> MMGHRPVLVLSQNTKRESGRKVQSGNINAAKTIADIIRTCLGPKSMMKMLLDPMGGIVMTNDGNAILREIQVQHPAAKSMIEISRTQDEEVGDGTTSVIILAGEMLSVAEHFLEQQMHPTVVISAYRKALDDMISTLKKISIPVDISDSDMMLNIINSSITTKAISRWSSLACNIALDAVKMVQFEENGRKEIDIKKYARVEKIPGGIIEDSCVLRGVMINKDVTHPRMRRYIKNPRIVLLDSSLEYKKGESQTDIEITREEDFTRILQMEEEYIQQLCEDIIQLKPDVVITEKGISDLAQHYLMRANITAIRRVRKTDNNRIARACGARIVSRPEELREDDVGTGAGLLEIKKIGDEYFTFITDCKDPKACTILLRGASKEILSEVERNLQDAMQVCRNVLLDPQLVPGGGASEMAVAHALTEKSKAMTGVEQWPYRAVAQALEVIPRTLIQNCGASTIRLLTSLRAKHTQENCETWGVNGETGTLVDMKELGIWEPLAVKLQTYKTAVETAVLLLRIDDIVSGHKKKGDDQSRQGGAPDAGQE;> MQDPNADTEWNDILRKKGILPPKESLKELEEEAEEEQRILQQSVVKTYEDMTLEELEDHEDEFNEEDERAIEMYRRRRLAEWKATKLKNKFGEVLEISGKDYVQEVTKAGEGLWVILHLYKQGIPLCALINQHLSGLARKFPDVKFIKAISTTCIPNYPDRNLPTIFVYLEGDIKAQFIGPLVFGGMNLTRDELEWKLSESGAIMTDLEENPKKPIEDVLLSSVRRSVLMKRDSDSEGD

ATP-dependent chaperonin TRiC/CCT partners with cochaperones prefoldin (PFD) and phosducin-like proteins (PhLPs) to facilitate folding of essential eukaryotic proteins. The ring-shaped chaperonin TCP-1 ring complex (TRiC, also called CCT) is a ~1 MDa hetero-oligomeric complex that has a double-chamber architecture, with each octameric ring formed by subunits CCT1-81–3. TRiC-mediated protein folding depends on an ATP-driven conformational cycle, which regulates the opening and closing of a built-in lid over the central chamber of each ring.

However, we could not detect any density attributable to the NTD. We, therefore, performed focused 3D classification on each CCT subunit. This analysis resolved an extended helical density that can be attributed to helix 3 (H3) of the NTD of PhLP2A adopting two different orientations associated with either the apical domain of CCT3 or CCT4. Notably, only the apical domains of CCT3 and CCT4 were predicted to form a dimeric complex with H3 of PhLP2A with good prediction scores, in agreement with our cryoEM density maps. The NTD of PhLP2A can adopt two different orientations, whereby H3 of the NTD contacts the apical regions of either CCT3 or CCT4. While the NTD is mostly negatively charged, H3 has a unique positively charged patch (residue 75–78), which displays a high degree of complementary to the negatively charged apical domains of CCT3 and CCT4 (Fig. 2a(i, ii), b). Mapping these crosslinks onto a predicted model of full-length PhLP2A suggests the NTD bends to place H1/H2 in the proximity of TXD. In good agreement with our PhLP2A-TRiC, we detected many intermolecular crosslinks between PhLP2A H3 and CCT3-CCT4 as well as between the PhLP2A TXD and CTD domains to the equatorial domains of CCT3 and CCT6 respectively (Fig. 1g(i, ii)). In the open state, the PhLP2A NTD adopts an H3 extended conformation to apical domains either CCT3 or 4.> ERDYPFFYKVGDLAGESNQVRWFLNVNLNKSDVTEDISIADRQGSGQQLNKESFTFDIVNDKETKYISLAEFEQQGYGKIDFVTDND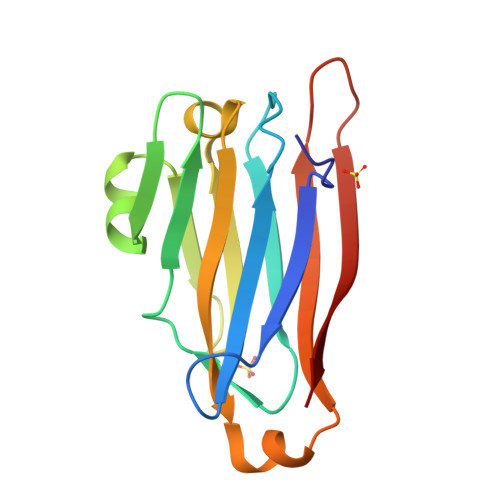FNLRFYRDKARFTSFIVRYTSTITEAGQHQATFENSYDINYQLNNQDATNEKNTSQVKNV> MIINEKYPYLSYLLRCYFNQDFEVLFGNADETLAAYKATETAEERLQMKAEIDYLLALSLPDDELQDILLNKLDCSYYYPNEWSSSEEWLKHIYKQMNHHHHH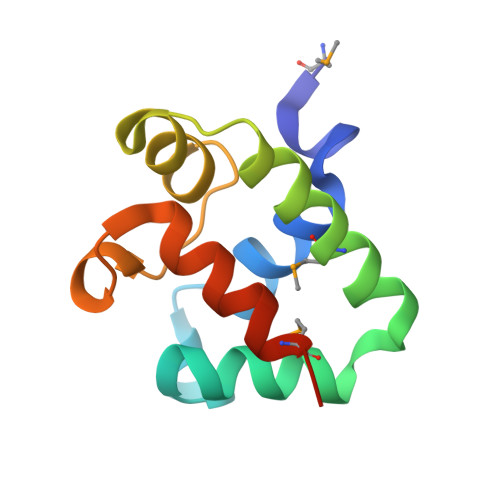H> MELKASISDYTEAEFLQLVTTICNADTSSEEELVKLVTHFEEMTEHPSGS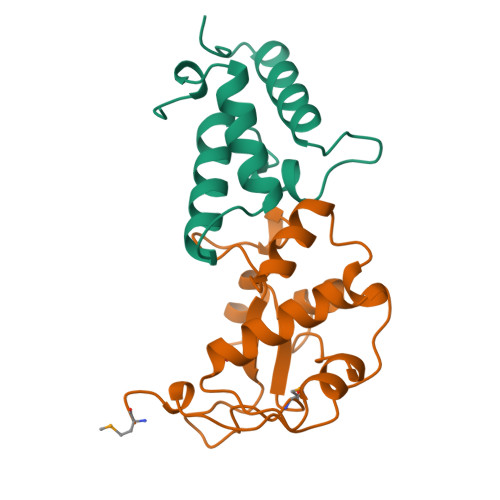DLIYYPKEGDDDSPSGIVNTVQQWRAANGKSGFKQG;> MESKRNKPGKATGKGKPVGDKWLDDAGKDSGAPIPDRIADKLRDKEFKSFDDFRKAVWEEVSKDPELSKNLNPSNKSSVSKGYSPFTPKNQQVGGRKVYELHHDKPISQGGEVYDMDNIRVTTPKRHIDIHRGK(2S)-N-[(4-carbamimidoylphenyl)methyl]-2-[[(2R,3R)-3-methyl-2-(phenylmethylsulfonylamino)pentanoyl]amino]pentanediamide 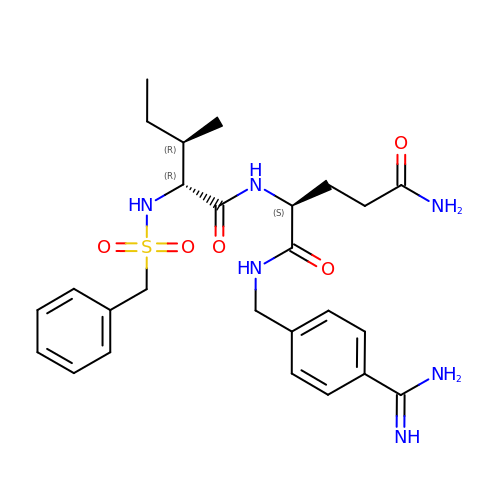| C26 H36 N6 O5 S | RKXCEYZSZWJMTQ-FRGLQRNOSA-N> QNSLALHKVIMVGSGGVGKSALTLQFMYDEFVEDYEPTKADSYRKKVVLDGEEVQIDILDTAGLEDYAAIRDNYFRSGEGFL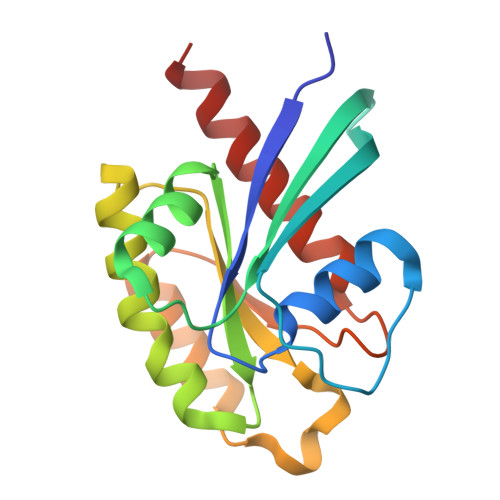CVFSITEMESFAATADFREQILRVKEDENVPFLLVGNKSDLEDKRQVSVEEAKNRAEQWNVNYVETSAKTRANVDKVFFDLMREIRARKMEDS>MGGSHHHHHHENLYFQGKKHTGYVGLKNQGATCYMNSLLQTLFFTNQLRKAVYMMPTEGDDSSKSVPLALQRVFYELQHSDKPVGTKKLTKSFGWETLDSFMQHDVQELCRVLLDNVENKMKGTCVEGTIPKLFRGKMVSYIQCKEVDYRSDRREDYYDIQLSIKGKKNIFESFVDYVAVEQLDGDNKYDAGEHGLQEAEKGVKFLTLPPVLHLQLMRFMYDPQTDQNIKINDRFEFPEQLPLDEFLQKTDPKDPANYILHAVLVHSGDNHGGHYVV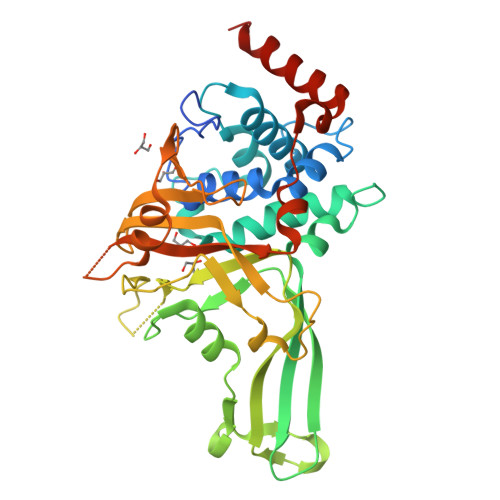YLNPKGDGKWCKFDDDVVSRCTKEEAIEHNYGGHDDDLSVRHCTNAYMLVYIRESKLSEVLQAVTDHDIPQQLVERLQEEKRIEAQKRKERQE[2x]>[6x]GTSSMADIGSKYLTRTRDIGANKKVDDLFGSASWETEEKMIKAKLITPNNKKRAFDKREVIVGRRGL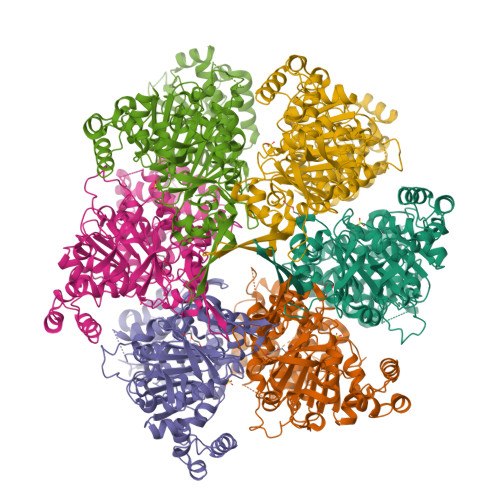GDFIAYAGQAFIGLIAPTRSGKGVGFIMPNMINYPQNIVVFDPKADTMETCGKIREKRFNQKVFIYEPFSLKTHRFNPFAYVDFGNDVVLTEDILSQIDTRLKGHGMVASGGDFSTQIFGLAKLVFPERPNEKDPFFSNQARNLFVINCNIYRDLMWTKKGLEFVKRKKIIMPETPTMFFIGSMASGINLIDEDTNMEKVVSLMEFFGGEEDKSGDNLRVLSPATRNMWNSFKTMGGARETYSSVQGVYTSAFAPYNNAMIRNFTSANDFDFRRLRIDEVSIGVIANPKESTIVGPILELFFNVMIYSNLILPIHDPQCKRSCLMLMDEFTLCGYLETFVKAVGIMAEYNMRPAFVFQSKAQLENDPPLGYGRNGAKTILDNLSLNMYYGINNDNYYEHFEKLSKVLGKYTRQDVSRSIDDNTGKTNTSISNKERFLMTPDELMTMGDELIILENTLKPIKCHKALYYDDPFFTDELIKVSPSLSKKYKLGKVPNQATFYDDLQAAKTRGELSYDKSLVPVGSSEL> GSHMASMKKKGSVVIVGRINLSGDTAYAQQTRGEEGCQETSQTGRDKNQVEGEVQIVSTATQTFLATSINGVLWTVYHGAGTRTIASPKGPVTQMYTNVDKDLVGWQAPQGSRSLTPCTCGSSDLYLVTRHADVIPVRRRGDSRGSLLSPRPISYLKGSSGGPLLCPAGHAVGIFRAAVSTRGVAKA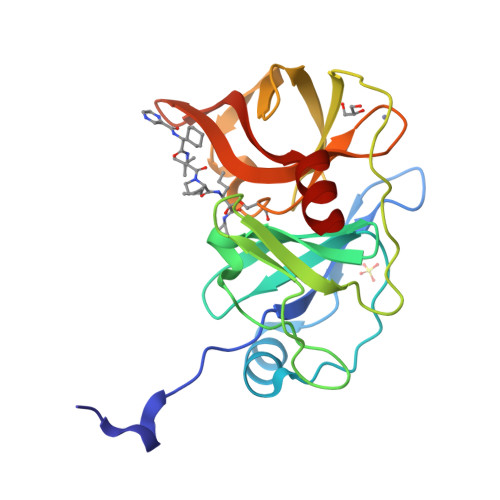VDFIPVESLETTMRSP>[7x]TNTLPHVAFYISVNRAISDEECTFNNSWLWKNEKGSRPFCKDANISLIYRVNLERSLQYGIVGSATPDAKIVRISLDDDSTGAGIHLNDQLGYRQFGASYTTLDAYFREWSTDAIAQDYRFVFNASNNKAQILKTFPVDNINEKFERKEVSGFELGVTGGVEVSGDGPKAKLEARASYTQSRWLTYNTQDYRIERNAKNAQAVSFTWNRQQYATAESLLNRSTDALWVNTYPVDVNRISPLSYASFVPKMDVIY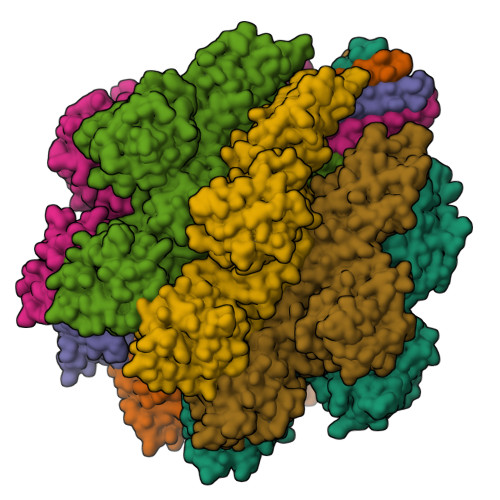KASATETGSTDFIIDSSVNIRPIYNGAYKHYYVVGAHQSYHGFEDTPRRRITKSASFTVDWDHPVFTGGRPVNLQLASFNNRCIQVDAQGRLTANMCDSQQSAQSFIYDQLGRYVSASNTKLCLDGAALDALQPCNQNLTQRWEWRKGTDELTNVYSGESLGHDKQTGELGLYASSNDAVSLRTITAYTDVFNAQESSPILGYTQGKMNQQRVGQDNRLYVRAGAAIDALGSASDLLVGGNGGSLSSVDLSGVKSITATSGDFQYGGQQLVALTFTYQDGRQQTVGSKAYVTNAHEDRFDLPDAAKITQLKIWADDWLVKGVQFDLN>GAHMAGRSMQAARCPTDELSLSNCAVVSEKDYQSGQHVIVRTSPNHKYIFTLRTHPSVVPGSVAFSLPQRKWAGLSIGQEIEVALYSFDKAKQCIGTMTIEIDFLQKKNIDSNPYDTDKMAAEFIQQFNNQAFSVGQQLVFSFNDKLFGLLVKDIEAMDPSILKGEPASGKRQKIEVGLVVGNSQVAFEKAENSSLNLIGKAKTKENRQSIINPDWNFEKMGIGGLDKEFSDIFRRAFASRVFPPEIVEQMGCKHVKGILLYGPPGCGKTLLARQIGKMLNAREPKVVNGPEILNKYVGESEANIRKLFADAEEEQRRLGANSGLHIIIFDEIDAICKQRGSMAGSTGVHDTVVNQLLSKIDGVEQLNNILVIGMTNRPDLIDEALLRPGRLEVKMEIGLPDEKGRLQILHIHTARMRGHQLLSADVDIKELAVETKNFSGAELEGLVRAAQSTAMNRHIKASTKVEVDMEKAESLQVTRGDFLASLENDIKPAFGTNQEDYASYIMNGIIKWGDPVTRVLDDGELLVQQTKNSDRTPLVSVLLEGPPHSGKTALAAKIAEESNFPFIKICSPDKMIGFSETAKCQAMKKIFDDAYKSQLSCVVVDDIERLLDYVPIGPRFSNLVLQALLVLLKKAPPQGRKLLIIGTTSRKDVLQEMEMLNAFSTTIHVPNIATGEQLLEALELLGNFKDKERTTIAQQVKGKKVWIGIKKLLMLIEMSLQMDPEYRVRKFLALLREEGASPLDFD[6x];>GSMDTSGKQAEAMALLAEAERKVKNSQSFFSGLFGGSSKIEEACEIYARAANMFKMAKNWSAAGNAFCQAAQLHLQLQSKHDAATCFVDAGNAFKKADPQEAINCLMRAIEIYTDMGRFTIAAKHHISIAEIYETELVDVEKAIAHYEQSADYYKGEESNSSANKCLLKVAGYAAQLEQYQKAIDIYEQVGTSAMDSPLLKYSAKDYFFKAALCHFCIDMLNAKLAVQKYEELFPAFSDSRECKLMKKLLEAHEEQNVDSYTESVKEYDSISRLDQWLTTMLLRIKKTIQGDEEDLR[4x];> GSNRRLQQTQAQVDEVVDIMRVNVDKVLERDQKLSELDDRADALQAGASQFETSAAKLKRKYW;> MALSEIETRHSEIIKLENSIRELHDMFMDMAMLVESQGEMIDRIEYNVEHAVDYVERAVSDTKKAVK;> RADQLADESLESTRRMLQL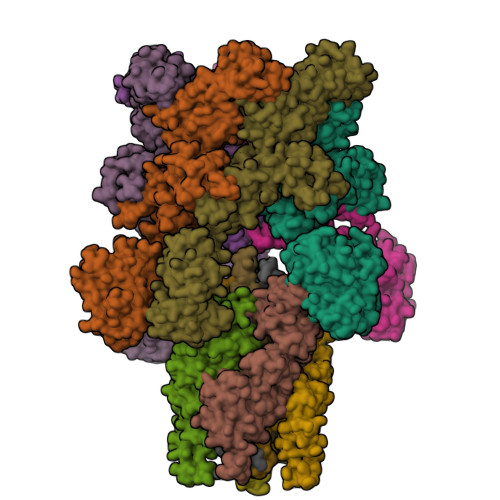VEESKDAGIRTLVMLDEQGEQLDRVEEGMNHINQDMKEAEKNLKDLGKFCGLCVCPCNKLKSSDAYKKAWGNNQDGVVASQPARVVDEREQMAISGGFIRRVTNDARENEMDENLEQVSGIIGNLRHMALDMGNEIDTQNRQIDRIMEKADSNKTRIDEANQRATKMLG Subclass B3 PBP (known as PBP3 in Escherichia coli and encoded by the ftsI gene) is active during cell division and localizes to a multiprotein complex termed the divisome, where it functions in PG synthesis in concert with the division-specific glycosyltransferase FtsW. PBP3 consists of three major domains: the N-terminal transmembrane helix anchors the protein in the cell membrane, while the C-terminal transpeptidase domain (TPd) is the catalytic module of PBP3 and mediates cross-linking of PG chains by ω-peptide linkages between d-Ala and meso-diaminopimelic acid (m-DAP) residues on opposing peptide chains. The catalytic serine acting as a nucleophile in the transpeptidation mechanism is also able to react with β-lactam antibiotics because of their structural similarity with the d-Ala-d-Ala motif; the resulting covalent intermediate, however, has a very long half-life (with turn-over constant k3 ~ 10−4 M−1s−1 or less), effectively leading to irreversible inactivation. AiCuris previously reported on the development of a novel monobactam (AIC499), which shows remarkable inhibitory activity against PBPs of Gram-negative bacteria, and good antibacterial activity, even against clinical isolates harboring several β-lactamase classes.

For E. coli PBP3, a soluble version of the P. aeruginosa orthologue was produced lacking the N-terminal transmembrane helix (PaPBP3ΔTM). Remarkably, three distinct crystal forms were identified for PaPBP3ΔTM, featuring different unit cells and lattice contacts but all belonging to space group C 1 2 1. Diffraction quality was generally superior when compared to EcPBP3ΔTM crystals, with moderate anisotropy and usable resolutions of 2.2 Å (crystal form 1), 1.8 Å (crystal form 2), and 1.9 Å (crystal form 3; for details refer to Table 1). In fact, the head subdomain (T77-R152) appears to largely bend as a rigid body, leading to slightly different orientations. These can be explained by packing effects; in addition to a lattice contact shared by all three structures (α1n-α2n region and α3n helix with the α2-β2a loop and the proximal α10 helix of a symmetry mate), crystal forms 1 and 3 feature unique interactions involving, among others, the α3n helix and β3n-α4n regions, respectively, contacting the β2e-β2f and α2-β2a segments, or the β2b-β2c hairpin, of neighboring molecules. In fact, the final models for crystal forms 2 and 3 lack several side chains in this region as well as small portions of the extreme N-terminus because of missing electron density, whereas in crystal form 1, larger parts of the backbone could not be traced. In the TPd, the largest differences between the three apo-PaPBP3ΔTM structures concern the β3-β4 and β5-α11 regions, both of which show indications of high flexibility. In crystal forms 1 and 2, eight and six residues are not resolved, respectively, while in crystal form 3 nine residues are missing.

> MDHDFLKGQGDARSVRHIAIPAHRGLITDRNGEPLAVSTPVTTLWANPKELMTAKERWPQLAAALGQDTKLFADRIEQNAEREFIYLVRGLTPEQGEGVIALKVPGVYSIEEFRRFYPAGEVVAHAVGFTDVDDRGREGIELAFDEWLAGVPGKRQVLKDRRGRVIKDVQVTKNAKPGKTLALSIDLRLQYLAHRELRNALLENGAKAGSLVIMDVKTGEILAMTNQPTYNPNNRRNLQPAAMRNRAMIDVFEPGSTVKPFSMSAALASGRWKPSDIVDVYPGTLQIGRYTIRDVSRNSRQLDLTGILIKSSNVGISKIAFDIGAESIYSVMQQVGLGQDTGLGFPGERVGNLPNHRKWPKAETATLAYGYGLSVTAIQLAHAYAALANDGKSVPLSMTRVDRVPDGVQVISPEVASTVQGMLQQVVEAQGGVFRAQVPGYHAAGKSGTARKVSVGTKGYRENAYRSLFAGFAPATDPRIAMVVVIDEPSKAGYFGGLVSAPVFSKVMAGALRLMNVPPDNLPTAKLVPRG> MVPISPIETVPVKLKPGMDGPKVKQWPLTEEKIKALVEICTEMEKEGKISKIGPENPYNTPVFAIKKKDSTKWRKLVDFRELNKR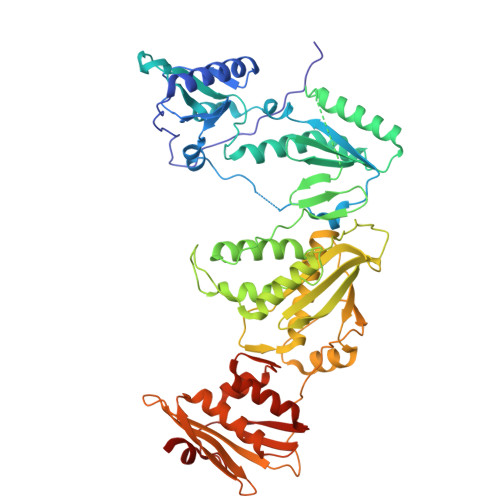TQDFWEVQLGIPHPAGLKKNKSVTVLDVGDAYFSVPLDEDFRKYTAFTIPSINNETPGIRYQYNVLPQGWKGSPAIFQSSMTKILEPFAAQNPDIVICQYMDDLYVGSDLEIGQHRTKIEELRQHLLRWGLTTPDKKHQKEPPFLWMGYELHPDKWTVQPIVLPEKDSWTVNDIQKLVGKLNWASQIYPGIKVRQLSKLLRGTKALTEVIPLTEEAELELAENREILKEPVHGVYYDPSKDLIAEIQKQGQGQWTYQIYQEPFKNLKTGKYARMRGAHTNDVKQLTEAVQKITTESIVIWGKTPKFKLPIQKETWETWWTEYWQATWIPEWEFVNTPPLVKLWYQLEKEPIVGAETFYVDGAANRETKLGKAGYVTNKGRQKVVPLTNTTNQKTELQAIYLALQDSGLEVNIVTDSQYALGIIQAQPDKSESELVNQIIEQLIKKEKVYLAWVPAHKGIGGNEQVDKLVSAG> D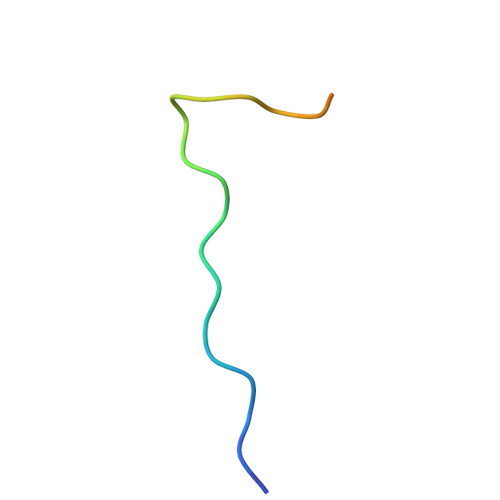RPPPYVAPPSYEGPHRTLGTKRGP> GGSMGKTADNHGPVRSETAREGRENQVYSPVTGARLVAGCICLTPDKKQVLMITSSAHKKRWIVPKGGVEKDEPNYETTAQRQTWEEAGCIGKIVANLGTVEDMRPPKDWNKDIKQFENSRKDSEVAKHPPRTEFHFYELEIENLLDKFPECHKRHRKLYSYTEAKQNLIDAKRPELLEALN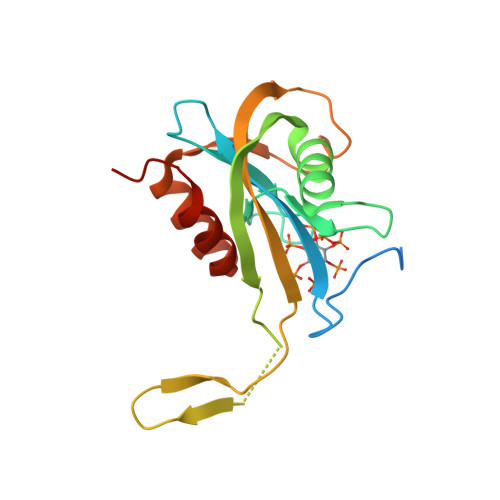RSAIIKDDK>[4x]GSMTEADVNPKAYPLADAHLTKKLLDLVQQSCNYKQLRKGANEATKTLNRGISEFIVMAADAEPLEIILHLPLLCEDKNVPYVFVRSKQALGRACGVSRPVIACSVTIKEGSQLKQQIQSIQQSIERLLV;>[4x]GPLGSEAAPEYRVIV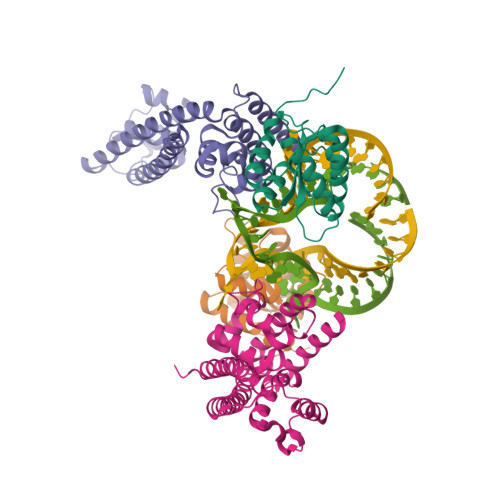DANNLTVEIENELNIIHKFIRDKYSKRFPELESLVPNALDYIRTVKELGNSLDKCKNNENLQQILTNATIMVVSVTASTTQGQQLSEEELERLEEACDMALELNASKHRIYEYVESRMSFIAPNLSIIIGASTAAKIMGVAGGLTNLSKMPACNIMLLGAQRKTLSGFSSTSVLPHTGYIYHSDIVQSLPPDLRRKAARLVAAKCTLAARVDSFHESTEGKVGYELKDEIERKFDKWQE> MDSQRSTLVHWFRKGLRLHDNPALSHIFTAANAAPGRYFVRPIFILDPGILDWMQVGANRWRFLQQTLEDLDNQLRKLNSRLFVVRGKPAEVFPRIFKSWRVEMLTFETDIEPYSVTRDAAVQKLAKAEGVRVETHCSHTIYNPELVIAKNLGKAPITYQKFLGIVEQLKVPKVLGVPEKLKNMPTPPKDEVEQKDSAA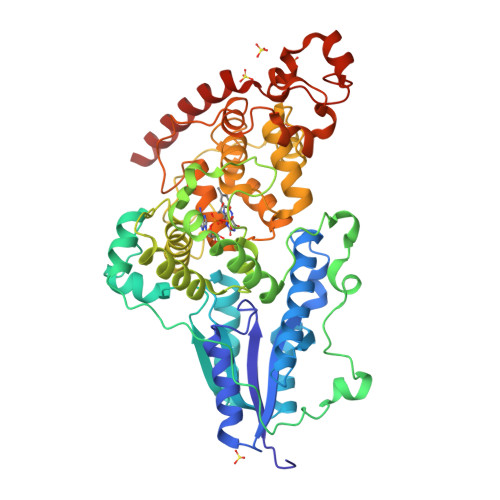YDCPTMKQLVKRPEELGPNKFPGGETEALRRMEESLKDEIWVARFEKPNTAPNSLEPSTTVLSPYLKFGCLSARLFNQKLKEIIKRQPKHSQPPVSLIGQLMWREFYYTVAAAEPNFDRMLGNVYCMQIPWQEHPDHLEAWTHGRTGYPFIDAIMRQLRQEGWIHHLARHAVACFLTRGDLWISWEEGQRVFEQLLLDQDWALNAGNWMWLSASAFFHQYFRVYSPVAFGKKTDPQGHYIRKYVPELSKYPAGCIYEPWKASLVDQRAYGCVLGTDYPHRIVKHEVVHKENIKRMGAAYKVNR> MHHHHHHLVPRGSVSKRDKRI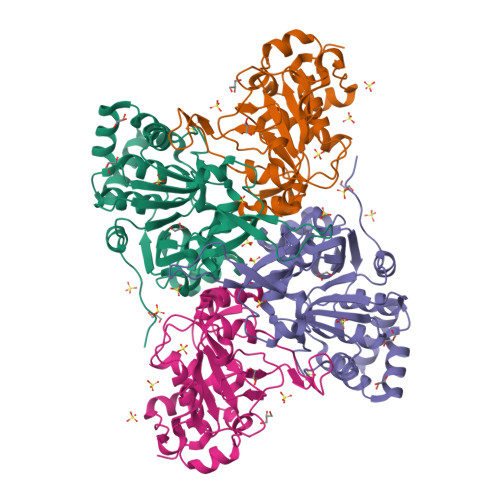SLDDAVGELRSGMTIGIGGWGSRRKPMALVRALLRSDVTDLTVVTYGGPDLGLLCSAGKVTKAYYGFVSLDSAPFYDPWFAKARTAGEIAVREMDEGMVKCGLEAAAARLPFLPIRAGLGSDVRRFWGDELRTVTSPYPDASGKSETLIAMPALNLDAALVHLNLGDKHGNAAYTGVDPYFDDLYCAAAEKRFVSVERVVETEELVKTVPLQNLILNRMMVDGVVEAPNGAHFTLAGDSYGRDEKFQRHYAESAKTPQAWQQFVATYLSGSEDDYQAAVKKFAEEQA;> MSETITEVTRAEYCAIACADIFSGAGEIMASPMATLPLIGARLARLTTEPDLLITDGEALIFADTPAVGAKAPIEGWMPFRKVFDVVASGRRHVVMGANQIDRHGNQNLSAFGPLQQPTRQMFGVRGAPGNTINHPTSYWVGKHTSRVFCDTVDIVSGVGYDQIDPENPAYRFHHLHRVVSNLGVFDFGGPDHTFRALSLHPGVTADQVADNTSFEVAGLADAGVTREPTDEELRLIREVLDPRSLRDREVSV> LQDQYKEGIKVVDIDDPDMMVDSFTMPNISHSNIDYQTLLANSDHAKFTIEPGVLPVGIDTHTATDIYQTLIALNLDTTVNDCLDKLLNDECTESTRENALYDYYALQLLPLQKAVRGHVLQFEWHQNSLLTNTHPNFLSKIRNINVQDALLTNQLYKNHELLKLERKKTEAVARLKSMNKSAINQYNRRQDKKNKRLKFGHRLIATHTNLERDEQKRAEKKAKERLQALKANDEEAYIKLLDQTKDTRITHLLRQTNAFLDSLTRAVKDQQKYTKEMIDSHIKEASEEVDDLSMVPKMKDEEYDDDDDNSNVDYYNVAHRIKEDIKKQPSILVGGTLKDYQIKGLQWMVSLFNNHLNGILADEMGLGKTIQTISLLTYLYEMKNIRGPYLVIVPLSTLSNWSSEFAK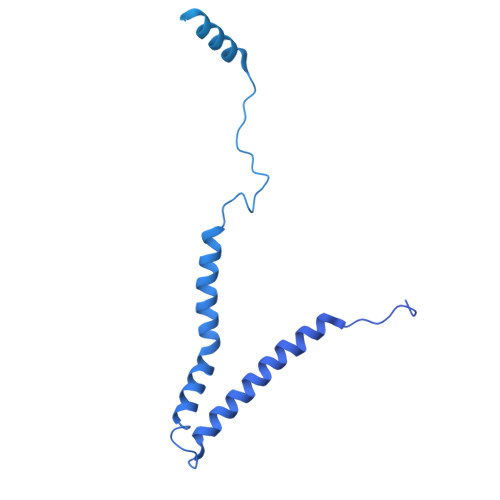WAPTLRTISFKGSPNERKAKQAKIRAGEFDVVLTTFEYIIKERALLSKVKWVHMIIDEGHRMKNAQSKLSLTLNTHYHADYRLILTGTPLQNNLPELWALLNFVLPKIFNSVKSFDEWFNTPFANTGGQDKIELSEEETLLVIRRLHKVLRPFLLRRLKKDVEKELPDKVEKVVKCKMSALQQIMYQQMLKYRRLFIGDQNNKKMVGLRGFNNQIMQLKKICNHPFVFEEVEDQINPTRETNDDIWRVAGKFELLDRILPKLKATGHRVLIFFQMTQIMDIMEDFLRYINIKYLRLDGHTKSDERSELLRLFNAPDSEYLCFILSTRAGGLGLNLQTADTVIIFDTDWNPHQDLQAQDRAHRIGQKNEVRILRLITTNSVEEVILERAYKKLDIDGKVIQAGKFDNKSTSEEQEALLRSLLDAEEERRKKRESGVEEEEELKDSEINEILARNDEEMAVLTRMDEDRSKKEEELGVKSRLLEKSELPDIYSRDIGAELKREESESAAVYNGRGARERKTATYNDNMSEEQWLRQFEVSDDEKNDKQARKQRTKKEDKSEAIDGGGSGGHHHHHH> MVAKGRIIRVTGPLVVADGMKGAKMYEVVRVGELGLIGEIIRLEGDKAVIQVYEETAGVRPGEPVVGTGASLSVELGPRLLTSIYDGIQRPLEVIREKTGDFIARGVTAPALPRDKKWHFIPKAKVGDKVVGGDIIGEVPETSIIVHKIMVPPGIEGEIVEIAEEGDYTIEEVIAKVKTPSGEIKELKMYQRWPVRVKRPYKEKLPP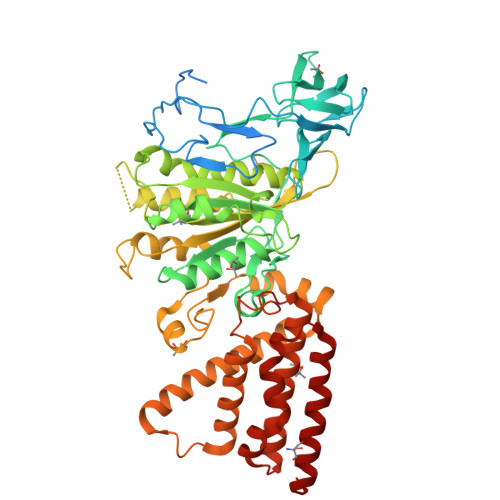EVPLITGQRVIDTFFPQAKGGTAAIPGPAGSGKTVTQHQLAKWSDAQVVIYIGCGERGNEMTDVLEEFPKLKDPKTGKPLMERTVLIANTSNMPVAAREASIYTGITIAEYFRDMGYDVALMADSTSRWAEALREISGRLEEMPGEEGYPAYLASKLAEFYERAGRVVTLGSDYRVGSVSVIGAVSPPGGDFSEPVVQNTLRVVKVFWALDADLARRRHFPAINWLTSYSLYVDAVKDWWHKNIDPEWKAMRDKAMALLQKESELQEIVRIVGPDALPERERAILLVARMLREDYLQQDAFDEVDTYCPPEKQVTMMRVLLNFYDKTMEAINRGVPLEEIAKLPVREEIGRMKFERDVSKIRSLIDKTNEQFEELFKKYGA>[3x]MAHHHHHHMSKTPLSIAHPWHGPVLTRDDYESLCCYIEITPADSVKFELDKETGILKVDRPQKFSNFCPCLYGLLPKTYCGDLSGEYSGQQSNR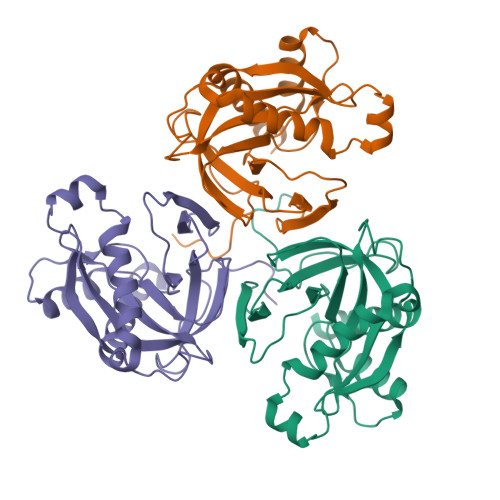ENIKGDGDPLDICVLTEKNITQGNILLQARPIGGIRILDSEEADDKIIAVLEDDLVYGNIEDISECPGTVLDMIQHYFLTYKATPESLIQAKPAKIEIVGLYGKKEAQKVIRLAHEDYCNLFM>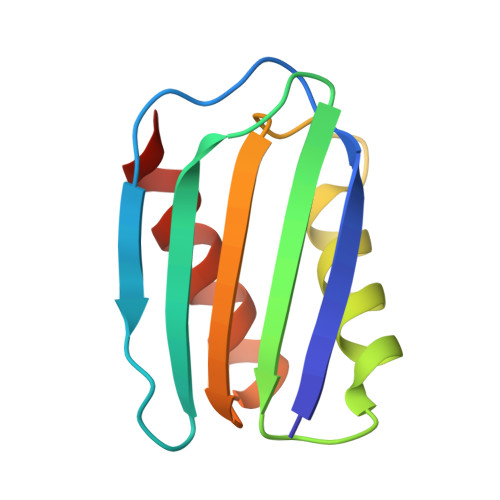 METLSFEFPAGQPGRGRALVGCVGSGDLEVLLEPGQPGKLSIQVQTSVNGSASRWQHLFERLFDGQTPPALLIDIHDFGATPGVVRLRLEQGFEEIGHD> YKLSKLRTSTIMTDYNPNYSFAGKTSSISDLKEVPRKNITLIRGLGHGAFGEVYEGQVSGMPNDPSPLQVAVKTLPEVCSEQDELDFLMEALIISKFNHQNIVRCIGVSLQSLPRFIL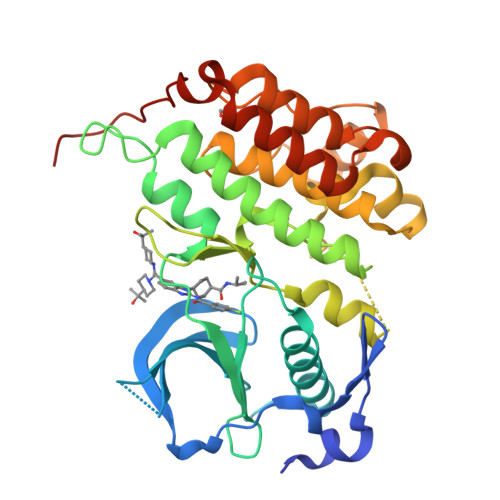LELMAGGDLKSFLRETRPRPSQPSSLAMLDLLHVARDIACGCQYLEENHFIHRDIAARNCLLTCPGPGRVAKIGDFGMARDIYRASYYRKGGCAMLPVKWMPPEAFMEGIFTSKTDTWSFGVLLWEIFSLGYMPYPSKSNQEVLEFVTSGGRMDPPKNCPGPVYRIMTQCWQHQPEDRPNFAIILERIEYCTQDPDVINTALPIEYGPLVEEEEK>[2x]SAKDLDAVDAILEQWRRERPDLDASPMGPIGRLRRCAVLMDQRLESCFSRFDLSSWEFDMLATLRRAGAPHCLSPTELFSTLM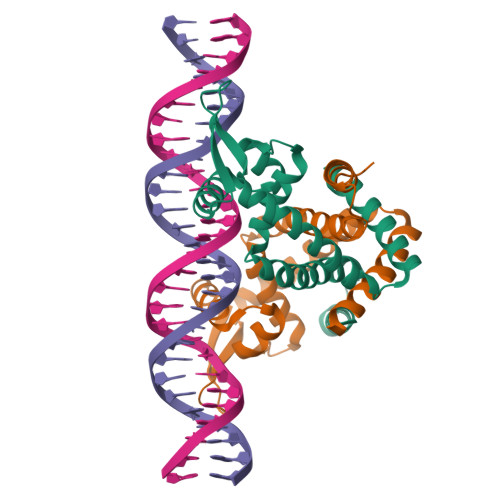VTSGTMTHRLKRLETRGFIERVQNELDARSTLVQLTSSGLELINRAVEAHIENERQVLSVLPAEVLAALDTNLAALLRGLESHNKGN>[4x]SNAWKQEELKFKTGLRRLQHRVGEIHLLREALQKGAEAGQVSLHSLIETPANGTGPSEALAMLLQETTGELEAAKALVLKRIQIWKRQQQLAGNGAPFEESLAPLQERCESLVDIYSQLQQEVGAAGGELEPKTRASLTGRLDEVLRTLVTSCFLVEKQPPQVLKTQTKFQAGVRFLLGLRFLGAPAKPPLVRADMVTEKQARELSVPQGPGAGAESTGEIINNTVPLENSIPGNCCSALFKNLLLKKIKRCERKGTESVTEEKCAVLFSASFTLGPGKLPIQLQALSLPLVVIVHGNQDNNAKATILWDNAFSEMDRVPFVVAERVPWEKMCETLNLKFMAEVGTNRGLLPEHFLFLA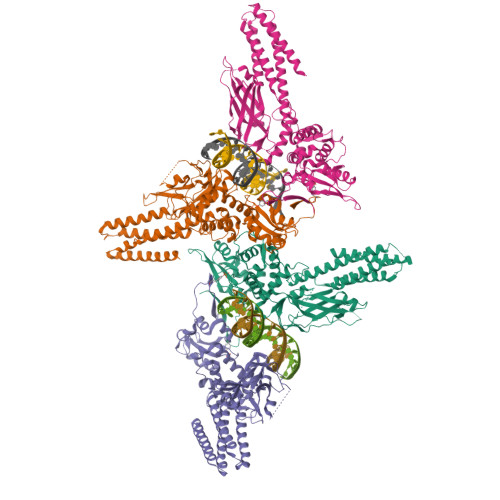QKIFNDNSLSMEAFQHRSVSWSQFNKEILLGRGFTFWQWFDGVLDLTKRCLRSYWSDRLIIGFISKQYVTSLLLNEPDGTFLLRFSDSEIGGITIAHVIRGQDGSPQIENIQPFSAKDLSIRSLGDRIRDLAQLKNLYPKKPKDEAFRSHYKPEQMGKDGRGYVPATIKMTVERDQPLPT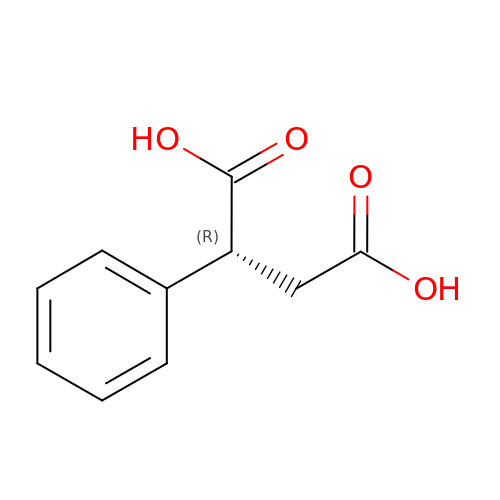(2R)-2-phenylbutanedioic acid | C10 H10 O4 | LVFFZQQWIZURIO-MRVPVSSYSA-N>AGDAEAGQGKVAVCGACHGVDGNSPAPNFPKLAGQGERYLLKQLQDIKAGSTPGAPEGVGRKVLEMTGMLDPLSDQDLEDIAAYFSSQKGSVGYADPALAKQGEKLFRGGKLDQGMPACTGCHAPNGVGNDLAGFPKLGGQHAAYTAKQLTDFREGNRTNDGDTMIMRG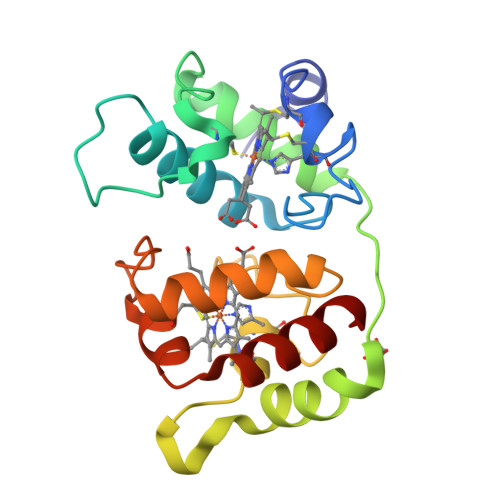VAAKLSNKDIEALSSYIQGLH[4x]>[2x]GDKFQLTFPLRTNY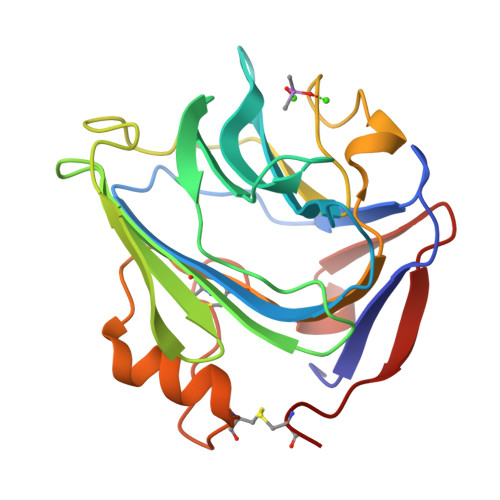MYAKVKKSLPEMYAFTVCMWLKSSATPGVGTPFSYAVPGQANELVLIEWGNNPMEILINDKVAKLPFVINDGKWHHICVTWTTRDGVWEAYQDGTQGGSGENLAPYHPIKPQGVLVLGQEQDTLGGGFDATQAFVGELAHFNIWDRKLTPGEVYNLATCSTKALSGNVIAWAESHIEIYGGATKWTFEACR>MIWKRKITLEALNAMGEGNMVGFLDIRFEHIGDDTLEATMPVDSRTKQPFGLLHGGASVVLAESIG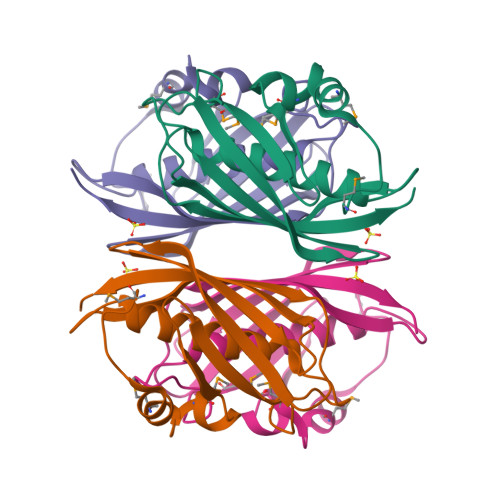SVAGYLCTEGEQKVVGLEINANHVRSAREGRVRGVCKPLHLGSRHQVWQIEIFDEKGRLCCSSRLTTAILLEHHHHHH[4x]> MLQFILRRLGLVIPTFIGITLLTFAFVHMIPGDPVMIMAGERGISPERHAQLLAELGLDKPMWQQYLHYIWGVMHGDLGISMKSRIPVWEEFVPRFQATLELGVCAMIFATAVGIPVGVLAAVKRGSIFDHTAVGLALTGYSMPIFWWGMMLIMLVSVHWNLTPVSGRVSDMVFLDDSNPLTGFMLIDTAIWGEDGNFIDAVAHMILPAIVLGTIPLAVIVRMTRSSMLEVLGEDYIRTARAKGLTRMRVIIVHALRNAMLPVVTVIGLQVGTLLAGAILTETIFSWPGLGRWLIDALQRRDYPVVQGGVLLVATMIILVNLLVDLLYGVVNPRIRHKK;> MSQVTENKVISAPVPMTPLQEFWHYFKRNKGAVVGLVYVVIVLFIAIFANWIAPYNPAEQFRDALLAPPAWQEGGSMAHLLGTDDVGRDVLSRLMYGARLSLLVGCLVVVLSLIMGVILGLIAGYFGGLVDNIIMRVVDIMLALPSLLLALVLVAIFGPSIGNAALALTFVALPHYVRLTRAAVLVEVNRDYVTASRVAGAGAMRQMFINIFPNCLAPLIVQASLGFSNAILDMAALGFLGMGAQPPTPEWGTMLSDVLQFAQSAWWVVTFPGLAILLTVLAFNLMGDGLRDALDPKLKQ;> MALLNVDKLSVHFGDESAPFRAVDRISYSVKQGEVVGIVGESGSGKSVSSLAIMGLIDYPGRVMAEKLEFNGQDLQRISEKERRNLVGAEVAMIFQDPMTSLNPCYTVGFQIMEAIKVHQGGNKSTRRQRAIDLLNQVGIPDPASRLDVYPHQLSGGMSQRVMIAMAIACRPKLLIADQPTTALDVTIQAQIIELLLELQQKENMALVLITHDLALVAEAAHKIIVMYAGQVVETGDAHAIFHAPRHPYTQALLRALPEFAQDKERLASLPGVVPGKYDRPNGCLLNPRCPYATDRCRAEEPALNMLADGRQSKCHYPLDDAGRPTL;> MSTQEATLQQPLLQAIDLKKHYPVKKGMFAPERLVKALDGVSFNLERGKTLAVVGESGCGKSTLGRLLTMIEMPTGGELYYQGQDLLKHDPQAQKLRRQKIQIVFQNPYGSLNPRKKVGQILEEPLLINTSLSKEQRREKALSMMAKVGLKTEHYDRYPHMFSGGQRQRIAIARGLMLDPDVVIADQPVSALDVSVRAQVLNLMMDLQQELGLSYVFISHDLSVVEHIADEVMVMYLGRCVEKGTKDQIFNNPRHPYTQALLSATPRLNPDDRRERIKLSGELPSPLNPPPGCAFNARCRRRFGPCTQLQPQLKDYGGQLVACFAVDQDENPQR

In Gram-negative bacteria, the full Dpp transporter is composed of five subunits: two integral membrane proteins (DppB and DppC) that form a translocation pathway for substrates; two ATPases (DppD and DppF) that bind and hydrolyze ATP during transport and a periplasm-localized SBP (DppA) for substrate capture. The Dpp transporter is primarily responsible for importing dipeptides but also capable of inefficiently importing tri- and tetrapeptides into the cell. Different from those structurally and mechanistically well-characterized ABC exporters that solely consist of two variable transmembrane domains (TMDs) and two highly conserved nucleotide-binding domains (NBDs), the ABC peptide importers require an additional substrate-binding protein (SBP) that captures peptide substrates and delivers them to the translocator for function. Unlike the reported heterotrimeric Mycobacterium tuberculosis DppBCD translocator, the E. coli DppBCDF translocator is a heterotetramer, with a [4Fe-4S] cluster at the C-terminus of each ATPase subunit.

To achieve this, we mutated Glu179 (E179) of DppD and Glu187 (E187) of DppF, two key catalytic residues for ATP hydrolysis, into glutamine residues (DppDE179Q and DppFE187Q). These mutations prevent ATP hydrolysis without affecting ATP binding. By incubating the inert ATP analogs, AMPPNP or ATPγS, and Mg2+ with the complex for 30 min in ice prior to cryo-EM sample preparation, we determined the ATPγS (or AMPPNP)-bound structures of the mutant DppBCDE179QFE187Q. Structures reveal that both ATPγS-DppBCDF and AMPPNP-DppBCDF adopt an inward-facing conformation, nearly identical to that of apo-DppBCDF. The RMSD between the ATPγS-DppBCDF and apo-DppBCDF is only 0.27 Å for 1,112 aligned Cα atoms. Intriguingly, although sequence alignment and structure superposition indicate that DppD, similar to DppF, does possess functional ATP binding-and-hydrolysis motifs, ATP analogues are only bound with DppF but not DppD in both ATPγS-DppBCDF and AMPPNP-DppBCDF. In DppBCDF and ATPγS (or AMPPNP)-DppBCDF, the periplasmic scoop motif region in DppB is invisible due to its conformational flexibility without interacting partner. In this state, binding of a single ATP molecule to DppF in DppBCDF does not induce conformational changes, and DppBCDF does not consume intracellular ATP.> MNDYYTPVVSHRFMASFIFNRIPDPLDIRFQRISGLSRELQVTQYSEGGENARNNYLAEKIQH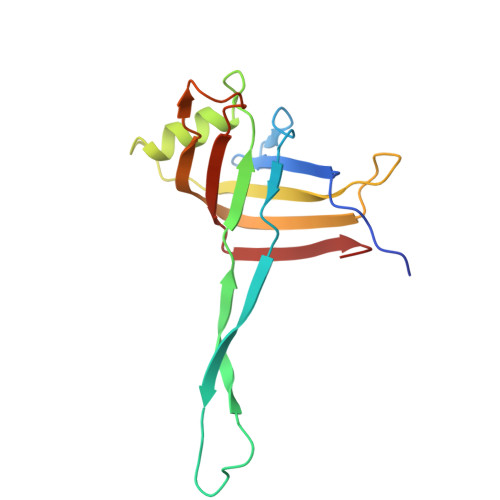GTLTLERGVMTVSPLTWMFDRVLSGEKIAYADVVVMLLNENSLPLSSWTLSNALPVRWQTSDFDANSNAILVNTLELRYQDMRWLGVKI>AMKIKIQKIHPNALIPKYQTDGSSGFDLHAVEEVMIKPHSVGLVKIGICLSLEVGYELQVRTRSGLALNHQVMVLNSPGTVDNDYRGEIKVILANLSDKDFKVQVGDRIAQGVVQKTYKAEFIECEQLDETSRGSGGFGST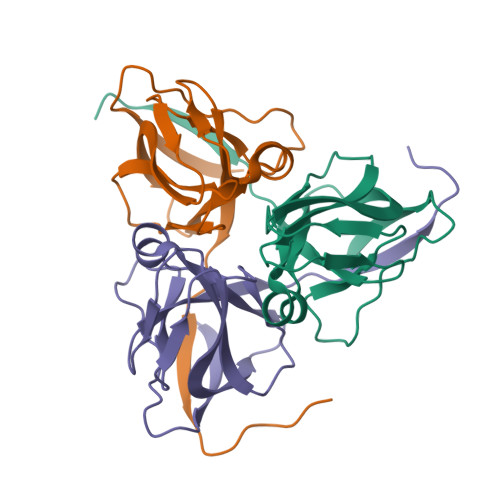GVSKAHHHHHH[3x]>DRSEATLIKRFKGEGVRYKAKLIGIDEVSAARGDKLCQDSMMKLKGVVAGARSKGEHKQKIFLTISFGGIKIFDEKTGALQHHHAVHEISYIAKDITDHRAFGYVCGKEGNHRFVAIKTAQAAEPVILDLRDLFQLIYELKQREELEKKAQKDKQCEQA[2x];>[2x]NGYE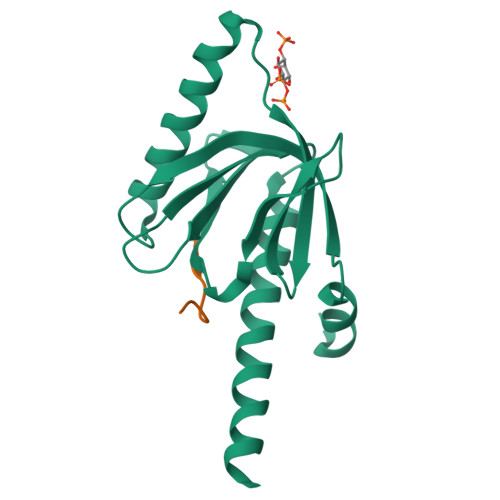NPTYK>MEALIPVINKLQDVFNTVGADIIQLPQIVVVGTQSSGKSSVLESLVGRDLLPRGTGIVTRRPLILQLVHVSQEDKRKTTGEENGVEAEEWGKFLHTKNKLYTDFDEIRQEIENETERISGNNKGVSPEPIHLKIFSPNVVNLTLVDLPGMTKVPVGDQPKDIELQIRELILRFISNPNSIILAVTAANTDMATSEALKISREVDPDGRRTLAVITKLDLMDAGTDAMDVLMGRVIPVKLGIIGVVNRSQLDINNKKSVTDSIRDEYAFLQKKYPSLANRNGTKYLARTLNRLLMHHIRDCLPELKTRINVLAAQYQSLLNSYGEPVDDKSATLLQLITKFATEYCNTIEGTAKYIETSELCGGARICYIFHETFGRTLESVDPLGGLNTIDILTAIRNATGPRPALFVPEVSFELLVKRQIKRLEEPSLRCVELVHEEMQRIIQHCSNYSTQELLRFPKLHDAIVEVVTCLLRKRLPVTNEMVHNLVAIELAYINTKHPDFADACGLMNNNIEEQRRNRLARELPSAVSRDKSSKVPSALAPASQEPSPAASAEADGKLIQDSRRETKNVASGGGGVGDGVQEPTTGNWRGMLKTSKAEELLAEEKSKPIPIMPASPQKGHAVNLLDVPVPVARKLSAREQRDCEVIERLIKSYFLIVRKNIQDSVPKAVMHFLVNHVKDTLQSELVGQLYKSSLLDDLLTESEDMAQRRKE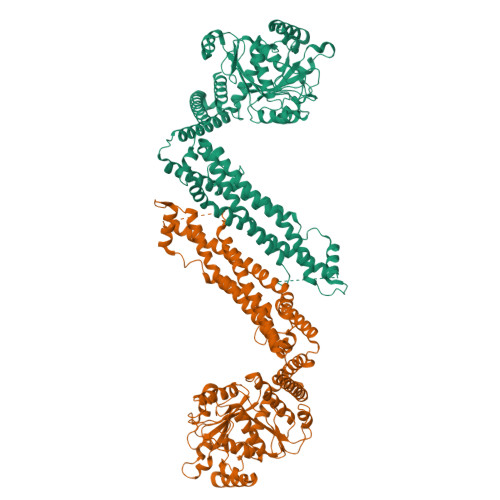AADMLKALQGASQIIAEIRETHLW[2x]>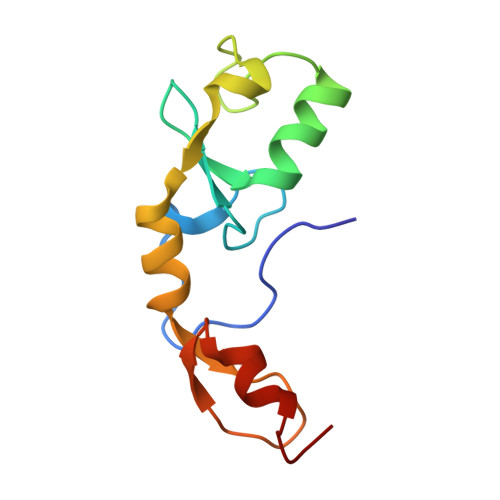 EIQGYDVEFDPPLESKYECPICLMALREAVQTPCGHRFCKACIIKSIRDAGHKCPVDNEILLENQLFPDNFAKREILSLMVKCPNEGCLHKMELRHLEDHQAHCEFA>QTLTLSPNLIGFNSNEGEKLLLTSRSREDFFPLSMQFVTQVNQAYCGVASIIMVLNSLGINAPETAQYSPYRVFTQDNFFSNEKTKAVIAPEVVARQGMTLDELGRLIASYGVKVKVNHASDTNIEDFRKQVAENLKQDGNFVIVNYLRKEIGQERGGHISPLAAYNEQTDRFLIMDVSRYKYPPVWVKTTDLWKAMNTVD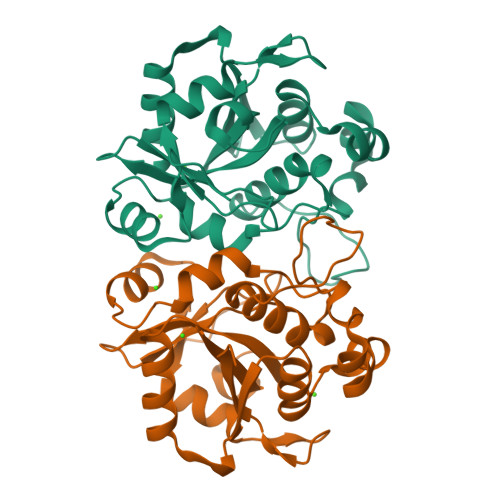SVSQKTRGFVFVSKTQD[2x]> MQSLTTALENLLRHLSQEIPATPGIRVIDIPFPLKDAFDALSWLASQQTYPQFYWQQRNGDEEAVVLGAITRFTSLDQAQRFLRQHPEHADLRIWGLNAFDPSQGNLLLPRLEWRRCGGKATLRLTLFSESSLQHDAIQAKEFIATLVSIKPLPGLHLTTT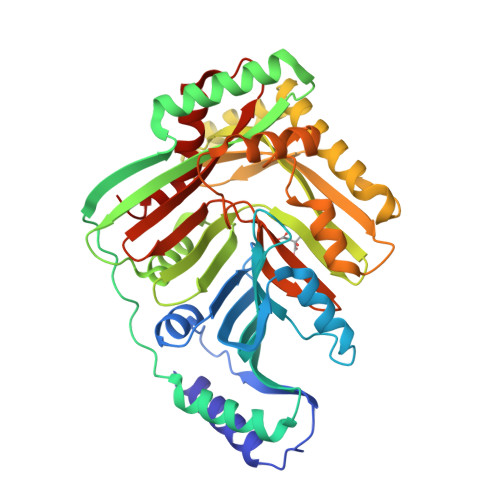REQHWPDKTGWTQLIELATKTIAEGELDKVVLARATDLHFASPVNAAAMMAASRRLNLNCYHFYMAFDGENAFLGSSPERLWRRRDKALRTEALAGTVANNPDDKQAQQLGEWLMADDKNQRENMLVVEDICQRLQADTQTLDVLPPQVLRLRKVQHLRRCIWTSLNKADDVICLHQLQPTAAVAGLPRDLARQFIARHEPFTREWYAGSAGYLSLQQSEFCVSLRSAKISGNVVRLYAGAGIVRGSDPEQEWQEIDNKAAGLRTLLQME>MTNAALDDKTIVRDYFNSTGFDRWRRIYGDGQVNFVQKDIRVGHQQTVDSVVAWLVADGNLPGLLVCDAGCGVGSLSIPLAQAGALVYGSDISEKMVGEAQQKAQEVLAYGNQPTFMTQDLAQLGGKYDTVICLDVLIHYPTEEASAMISHLASLADRRLILSFAPKTLGLTVLKKIGGLFPGPSKTTRAYQHKEADIRKILGDNGFSIARTGMTSTRFYYSRILEAVRSLEHH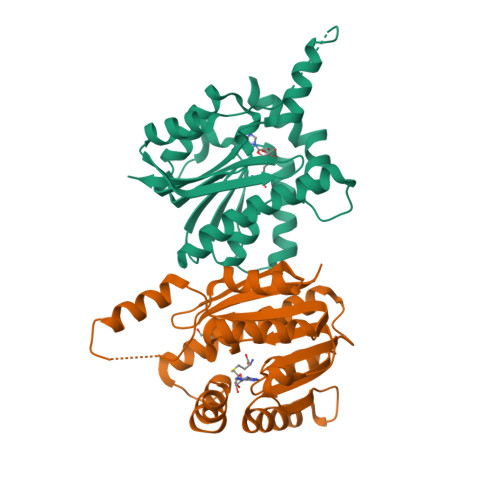HHHH[2x]>[3x]MGDGANSDAAKEYLTKDSFSYEVYGIIAMQAAYRDYDSGDAKQDDNLGGMQLNNESRIGFRGKKQFANFEPTFIWQIEGGYVDPSFGGEGAGLGERDTFVGFESASWGQVRLGRVLTPMYELVDWPASNPGLGDVYDWGGAIGGAKYQDRQSNTIRWDSPMYADKFSIDAAVGAGDKAGLGAGDDYWGGIAAHYKLGPLQLDAAYEGNRNIEAEGQTWENNTYLVGVQGWFENGISFFAQYKYMEADASNGVNEKQDAMSAGLMYTTGDWQYKLGYAANFDLERDGKTLSNTSDDVVSAQIMYFVDPSAVLYARARMNDFNEGLDGLDDAARWTSGTNGDYNEYSVGVEYYF

The gene encoding for ChiP is found in most marine members of the Vibrionaceae, emphasizing the general importance of this OM diffusion channel for chitin utilization. The addition of micromolar concentrations of chitooligosaccharides such as chitohexaose (GlcNAc6) causes a complete block of ionic current, demonstrating tight binding. Here, we report X-ray crystal structures of VhChiP in the absence and presence of chitooligosaccharides.

Subsequently we cloned VhChiP without a signal sequence and with a C-terminal His6-tag into pET28a to express the protein into inclusion bodies (IBs) and avoid toxicity issues. VhChiP from IBs was folded in vitro from 8 M urea and purified as the native protein. In vitro-folded VhChiP forms a trimeric assembly of oval β-barrels, each consisting of 16 strands, like the general diffusion porins OmpF/C from E. coli. Unlike OmpF/C however, the N-terminus of VhChiP does not form an intramolecular salt bridge with the C-terminal carboxyl group. Instead, the first N-terminal 17 amino acids of VhChiP are not part of the barrel and extend into the periplasm where they form a trimerization motif like that observed in the phosphate transporter OprP from Pseudomonas aeruginosa. The first nine amino acids of the N-terminus are disordered and not visible in the electron density. The N-terminal ten residues of in vitro-folded VhChiP are highly flexible and do not insert into the pore.Non-hydrolasable alarmone analogue | 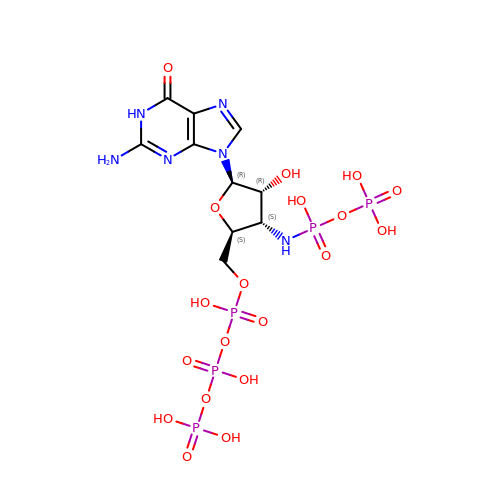C10 H19 N6 O19 P5 | IZNYESBVRGWINY-DXTOWSMRSA-N>MAHAGRTGYDNREIVMKYIHYKLSQRGYEWDAGDDVEENRTEAPEGTESEVVHLTLRQAVDDFSRRYRRDFAEMSSQLHLTPFTARGRFATVVEELFRDGVNWGRIVAFFEFGGVMCVESVNRE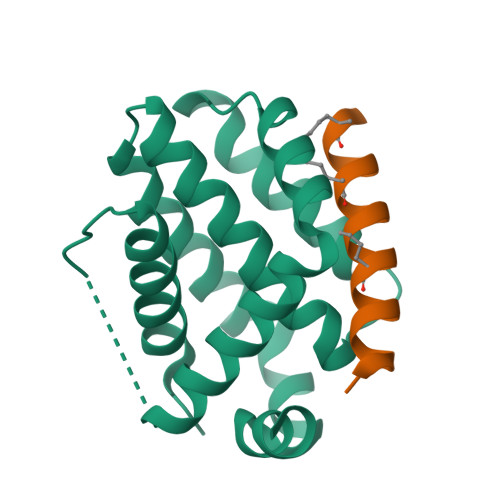MSPLVDNIALWMTEYLNRHLHTWIQDNGGWDAFVELYGPSMR[6x];>XWLAQRLGRELRRLSDEFVDSFK[8x]> GAGCACCTGTA;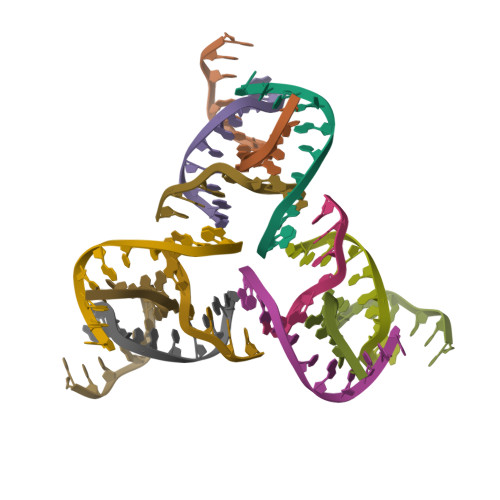> ACACCGT;> CCTGACTGTGGTGC;> CGGACAGTCA> KDIEISASE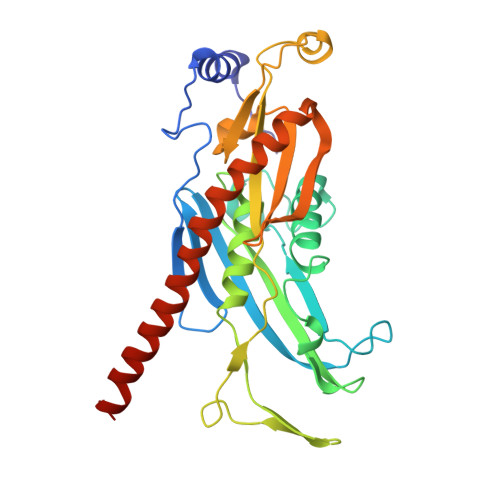SKFILEALRQNYRLDGRSFDQFRDVEITFGKEFGDVSVKMGNTKVHCRISCQIAQPYEDRPFEGLFVISTEISPMAGSQFENGNITGEDEVLCSRIIEKSVRRSGALDVEGLCIVAGSKCWAVRADVHFLDCDGGFIDASCIAVMAGLMHFKKPDITVHGEQIIVHPVNEREPVPLGILHIPICVTFSFFNPQDTEENIKGETNSEISIIDATLKEELLRDGVLTVTLNKNREVVQVSKAGGLPMDALTLMKCCHEAYSIIEKITDQILQLLKEDSEKRNKYAAMLTSENAREI>[3x]AP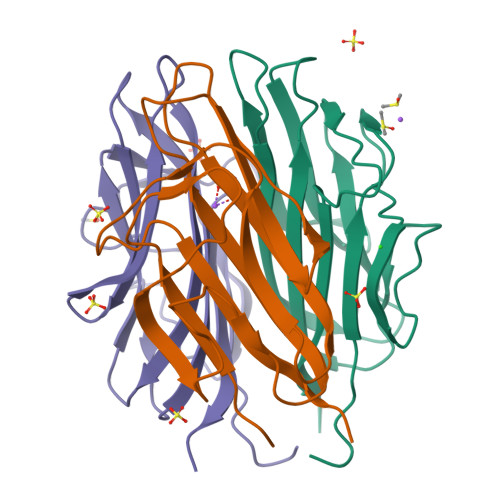GDPKIAFYAGLKRQHEGYEVLKFDDVVTNLGNHYDPTTGKFTCSIPGIYFFTYHVLMRGGDGTSMWADLCKNNQVRASAIAQDADQNYDYASNSVVLHLEPGDEVYIKLDGGKAHGGNNNKYSTFSGFIIYADAAA>MVDFKLSPSQLEARRHAQAFANTVLTKASAEYSTQKDQLSRFQATRPFYREAVRHGLIKAQVPIPLGGTMESLVHESIILEELFAVEPATSITIVATALGLMPVILCDSPSLQEKFLKPFISGEGEPLASLMHSEPNGTANWLQKGGPGLQTTARKVGNEWVISGEKLWPSNSGGWDYKGADLACVVCRVSDDPSKPQDPNVDPATQIAVLLVTRETIANNKKDAYQILGEPELAGHITTSGPHTRFTEFHVPHENLLCTPGLKAQGLVETAFAMSAALVGAMAIGTARAAFEEALVFAKSDTRGGSKHIIEHQSVADKLIDCK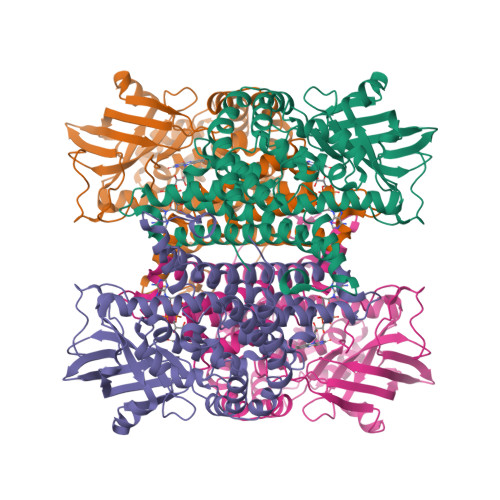IRLETSRLLVWKAVTTLEDEALEWKVKLEMAMQTKIYTTDVAVECVIDAMKAVGMKSYAKDMSFPRLLNEVMCYPLFDGGNIGLKRRQMQRVMALEDYEPWAATYGSSKVDKSRL[4x]> GSKQVITEQIANDLVKEVVNSSVISIVKREFSEANYRKDFIDTMTRELYDAFLHERLYLIYMDSRAELKRNSTLKKKFFEKWQ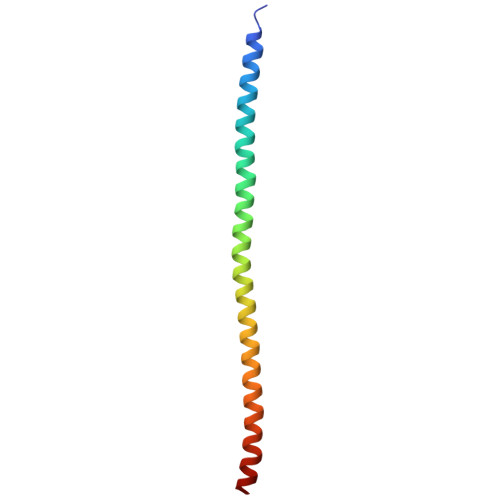AS> G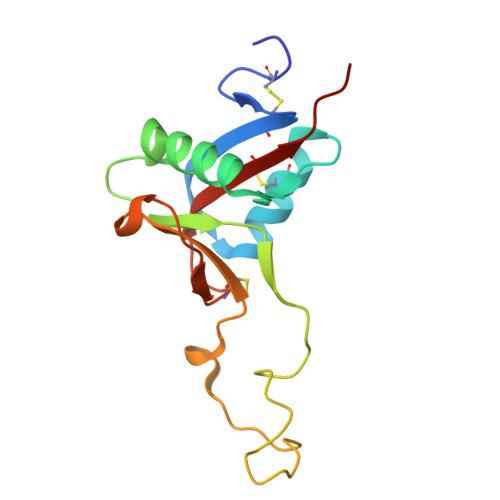LHCPSDWYYYDQHCYRIFNEEMNWEDAEWFCTKQAKGAHLVSIKSAKEADFVAWMVTQNIEESFSHVSIGLRVQNKEKQCSTKWSDGSSVSYDNLLDLYITKCSLLKKETGFRKWFVASCIGKIPFVCKFPPQC Four helix bundles are also attractive for synthetic chemists because its interfaces are dominated by side chain and side chain interactions, which can be more tunable than β-strands. This study focuses on TmFtn, a naturally dimeric protein consisting of two antiparallel four helix bundles, as shown in Supplementary Fig. 1. Thermotoga maritima ferritin (TmFtn) naturally occurs as a dimer; twelve of these dimers interact with each other in a head-to-side manner to generate 24-meric hollow protein nanocage in the presence of Ca2+ or PEG. By tuning two contiguous dimeric proteins to interact in a fully or partially side-by-side fashion through protein interface redesign, we can render the self-assembly transformation of such dimeric building blocks from the protein nanocage to filament, nanorod and nanoribbon in response to multiple external stimuli.

We made a mutant named FLAL where Asn147 was replaced by aromatic phenylalanine (Phe) residue to create π–π interactions, while Glu112, Glu113, and Lys114 were replaced by three hydrophobic residues Leu, Ala, and Leu to decrease the electrostatic repulsion and increase the hydrophobic interactions between two adjacent dimers at the same time. To confirm this idea, we examined the FLAL self-assembly behavior in solution concerning Ca2+ and FLAL concentrations. Upon screening the concentration of Ca2+ and FLAL, we found that the optimal condition for the formation of filaments is [FLAL] = 48.0 μM and [Ca2+] = 80.0 mM, which is close to the Ca2+ concentration (50 mM) used for the above nanocage assembly. To obtain detailed structural information on the FLAL filament, we tried to crystallize this protein and eventually obtained qualified single crystals suitable for X-ray diffraction. The crystal structure was solved at a resolution of 2.1 Å. The side view of the crystal structure revealed that FLAL molecules arrange in a repeating, side-by-side fashion to form filaments. Further crystal analyses reveal that two adjacent FLAL molecules have opposite orientations, forming another interface along their C and D helixes. In the structure with resolutions that permit detailed analysis of side-chain configurations, Phe147 and Leu114 side chains at the designed interface adopt suitable conformations to generate π–π stacking interactions and hydrophobic interactions, respectively, again approving our design at an atomic level. Besides the designed noncovalent interactions, Leu112 and Val119 also produce hydrophobic interactions, which is unexpected. Additionally, one calcium ion occurs nearby the designed protein interface, which binds to Glu108, Asp127, Asn105, and one water molecule. We believe that the cooperation of these noncovalent interactions and metal coordination along the inter-building-block interfaces promotes the formation of the filaments.

>[2x]MMVISEKVRKALNDQLNREIYSSYLYLSMATYFDAEGFKGFAHWMKKQAQEELTHAMKFYEYIYERGGRVELEAIEKPPSNWNGIKDAFEAALKHEEFVTQSIYNILELASLALDHATVSFLKWFVDEQVEEEDQVREILDLLEKAFGQMSVIFQLDRYLGQRE Toll-like Receptor 3 (TLR3) plays a key role in anti-viral defenses by inducing a potent immune response against double-stranded RNAs (dsRNAs) produced by viral infection. Previous crystallographic studies show that RNA ligand binds to the extracellular domains of TLR3 and induces the formation of a homodimer of TLR326. The charge interaction with the phosphate backbone of the RNA double helix plays the principal role in the interaction. The ligand-binding site involves both the N and C-terminal parts of the TLR3 ectodomain.

To determine whether the transmembrane and intracellular domains are necessary for the linear clustering of TLR3, we produced the ectodomain of TLR3 (ectoTLR3) and determined its structure in complex with poly(I:C) dsRNA. The electron micrographs show that the majority of the ectoTLR3s are in the clustered state. The structure of the ectoTLR3-dsRNA complex is not changed by the deletion mutation and is superimposable with that of the full-length TLR3-dsRNA complex with an r.m.s.d. of 0.42 Å. Interestingly, the C-terminal ends of the TLR3 ectodomains in the cluster point to the same direction even without the transmembrane and intracellular domains. This observation demonstrates that anchoring to the membrane is not necessary to fix the orientations of the transmembrane and intracellular domains in the cluster. Several factors can contribute to the ordered assembly of TLR3 along the dsRNA strands. First, as shown in Fig. 2, the deletion of both the transmembrane and the intracellular domains did not change the structure of the receptor cluster. Close inspection of the region between the TLR3 dimeric units in the cluster shows that the charge interaction plays a role in the clustering. The closest contact area between the dimeric TLR3 units is composed of the negatively charged N-terminal and the positively charged C-terminal residues of the neighboring ectoTLR3 dimers. The distance between these charged areas is more than 6 angstroms and appears too far to be considered a strong interaction.

>[4x]ADPKCTVSHEVADCSHLKLTQVPDDLPTNITVLNLTHNQLRRLPAANFTRYSQLTSLDVGFNTISKLEPELCQKLPMLKVLNLQHNELSQLSDKTFAFCTNLTELHLMSNSIQKIKNNPFVKQKNLITLDLSHNGLSSTKLGTQVQLENLQELLLSNNKIQALKSEELDIFANSSLKKLELSSNQIKEFSPGCFHAIGRLFGLFLNNVQLGPSLTEKLCLELANTSIRNLSLSNSQLSTTSNTTFLGLKWTNLTMLDLSYNNLNVVGNDSFAWLPQLEYFFLEYNNIQHLFSHSLHGLFNVRYLNLKRSFTKQSISLASLPKIDDFSFQWLKCLEHLNMEDNDIPGIKSNMFTGLINLKYLSLSNSFTSLRTLTNETFVSLAHSPLHILNLTKNKISKIESDAFSWLGHLEVLDLGLNEIGQELTGQEWRGLENIFEIYLSYNKYLQLTRNSFALVPSLQRLMLRRVALKNVDSSPSPFQPLRNLTILDLSNNNIANINDDMLEGLEKLEILDLQHNNLARLWKHANPGGPIYFLKGLSHLHILNLESNGFDEIPVEVFKDLFELKIIDLGLNNLNTLPASVFNNQVSLKSLNLQKNLITSVEKKVFGPAFRNLTELDMRFNPFDCTCESIAWFVNWINETHTNIPELSSHYLCNTPPHYHGFPVRLFDTSSCKSGRLVPRGSHHHHHH>ANIQSFSFKNFNSPSFILQG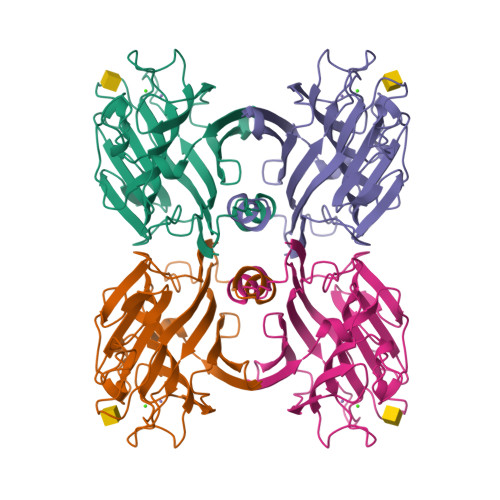DATVSSGKLQLTKVKENGIPTPSSLGRAFYSSPIQIYDKSTGAVASWATSFTVKISAPSKASFADGIAFALVPVGSEPRRNGGYLGVFDSDVYNNSAQTVAVEFDTLSNSGWDPSMKHIGIDVNSIKSIATVSWDLANGENAEILITYNAATSLLVASLVHPSRRTSYILSERVDITNELPEYVSVGFSATTGLSEGYIETHDVLSWSFASKLPDDSTAEPLDLASYLVRNVL[2x]>[3x]MTAKDDYPSLSFQQDYVYIFSSDFQLSEELGVALINALSAKEIVPERLYVMLNDKTISFSFISKNKKSKNRVL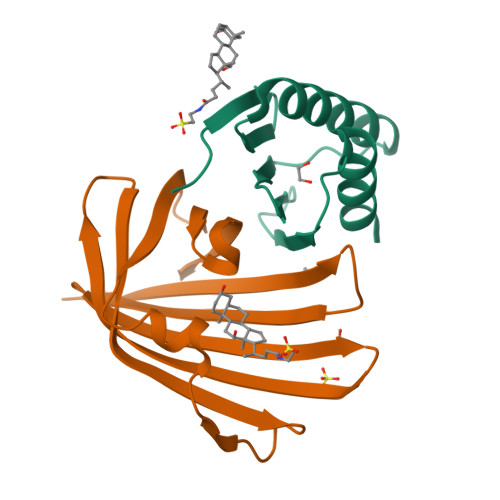STEKKLNYKHISEYIVNEIEY;>[3x]MGSSHHHHHHSQDPVHFYETSYKYQAADSTYMHDVAINVSIKGNHFTSDIIIRELVKSENKNYYNVIGHGDIIQKNTHQYYLNFDNIDVYTGTNKANMKPYKEPTSISSLINKSNNIRVVYLSEEYVVVEFFFYDGQIITLHRY>MRRGIAATALAASIALTATACGGSDSGDSAGGPVTLTWWDTSNATNEAPTYKALVKEFEAAHKDIKVKYVNVPFDQAQNKFDTAAGATGAPDILRSEVGWTPAFAKKGFFLPLDGTEALKDQDKFQPSLIKQAQYDGKTYGVPFVTDTLALVYNKQLFEKAGLTEAPRTWDDLKKAAATIKGKTGVDGYWGSTQAYYAQSFLYGDGTDTVDVPAKKITVNSPEAKKAYGTWLGLFDGKGLHKADTTADAYAHIQDAFVNGKVASIV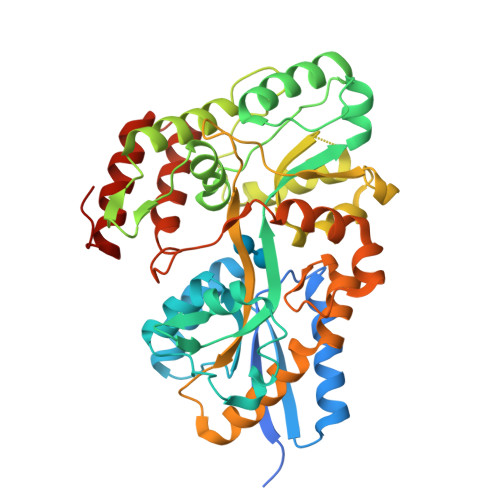QGPWEITNFYKGSAFKDKANLGIATVPAGTSGKAGAPTGGHNLSVYAGSDKAHQEASLKFIEFMTSAKSQETIALKNSTLPTRDDAYTAEVKADPGIAGYQTVLAAARPRPELPEYSSLWGPLDTELLAIAGGKESLDKGLGNAETAIAKLVPDYSKHHHHHH[2x]(3S)-3-({[(Z)-phenylmethylidene]carbamoyl}amino)-N-(1H-tetrazol-5-yl)-1-[3-(trifluoromethyl)benzoyl]-2,3-dihydro-1H-indole-3-carboxamide 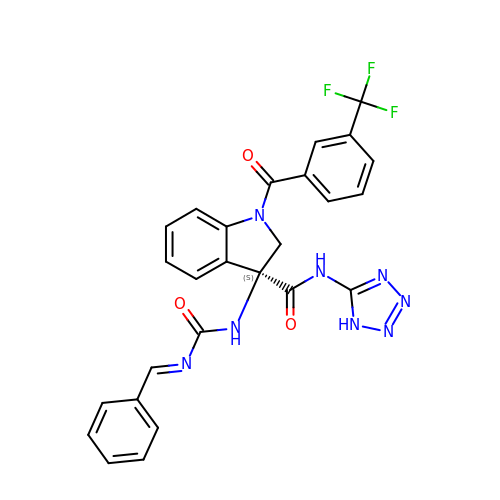| C26 H19 F3 N8 O3 | IOANIZJZIOBFFS-MDTWIARKSA-N> MAGASVKVAVRVRPFNSREMSRDSKCIIQMSGSTTTIVNPKQPKETPKSFSFDYSYWSHTSPEDINYASQKQVYRDIGEE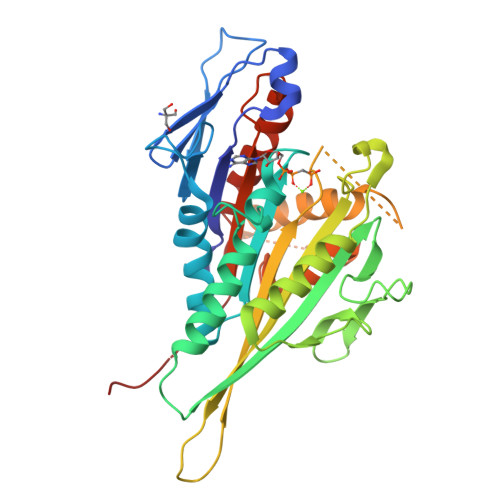MLQHAFEGYNVCIFAYGQTGAGKSYTMMGKQEKDQQGIIPQLCEDLFSRINDTTNDNMSYSVEVSYMEIYCERVRDLLNPKNKGNLRVREHPLLGPYVEDLSKLAVTSYNDIQDLMDSGNKARTVAATNMNETSSRSHAVFNIIFTQKRHDAETNITTEKVSKISLVDLAGSERADSTGAKGTRLKEGANINKSLTTLGKVISALAEMDSGPNKNKKKKKTDFIPYRDSVLTWLLRENLGGNSRTAMVAALSPADINYDETLSTLRYADRAKQIRNTVSVNHHHHH>GTIITVTAQANEKNTRTVSTAKGDKKIISVPLFEKEKGSNVKVAYGSAFLPDFIQLGDTVTVSGRVQAKESGEYVNYNFVFPTVE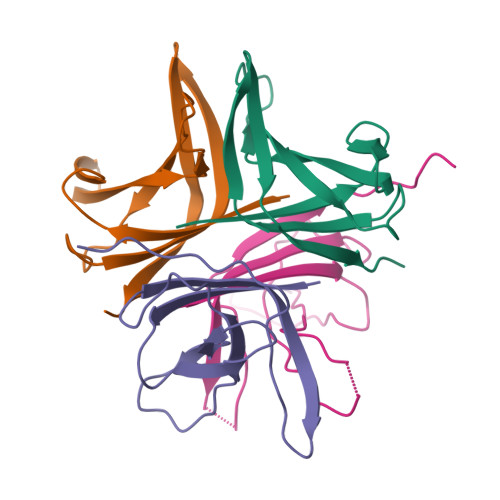KVFITNDNSSQSQAKQDLFGGSEPIEVNSEDLPF[4x]> KETAAAKFERQHMDSSTSAASSSNYCNQMMKSRNLTKDRCKPCNTFVHESLADVQAVCSQKNVACKNGQTNCYQSYSTMSITDCCETGSSKYPNCAYKTTQANKH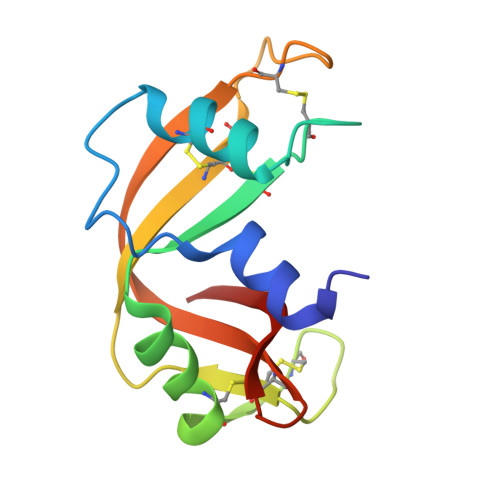IIVACEGNPYVPVHFDASV> MQQLNPSEISALIKQRIGDLDTSATAKNEGTIVMVSDGIVRIHGLADAMYGEMIEFDGGLFGMALNLEQDSVGAVVLGNYLSLQEGQKARCTGRVLEVPVGPELLGRVVDALGNPIDGKGPIDAKLTDAVEKVAPGVIWRQSVDQPVQTGYKSVDTMIPVGRGQRELIIGDRQTGKTAMAIDAIIAQKNSGIKCVYVAIGQKQSTIANVVRKLEETGAMAYTTVVAAAAADPAAMQYLAPYSGCTMGEYFRDRGEDALIIYDDLSKQAVAYRQISLLLRRPPGREAYPGDVFYLHSRLLERASRVSAEYVEKFTNGAVTGKTGSLTALPIIETQAGDVSAFVPTNVISITDGQIFLETSLFNAGIRPAVNAGISVSRVGGSAQTKIIKKLSGGIRTALAQYRELA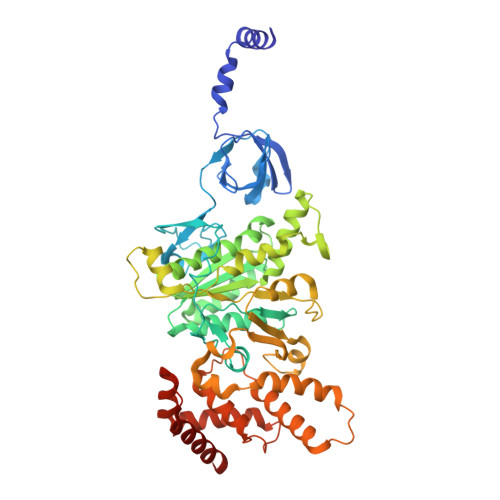AFAQFASDLDEATRKQLEHGQRVTELMKQKQYAPYSIADQAVSVYASNEGYMADVEVKKIVDFDAALIAYFRSEYAPLMKQIDETGDYNKDIEAAIKAGIESFKATQTY>[4x]CTAACCCT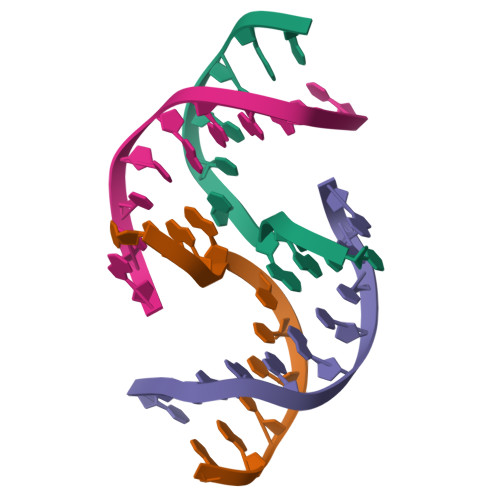AA;>TTAGGGTTAG[4x]>GAMGSKNWFKITIPYGRKYDKAWLLSMIQSKCSVPFTPIEFHYENTRAQFFVEDASTASALKAVNYKILDRENRRISIIINSSAPPHTILNELKPEQVEQLKLIMSKRYDGSQQALDLKGLRSDPDLVAQNIDVVLNRRSCMAATLRIIEENIPELLSLNLSNNRLYRLDDMSSIVQKAPNLKILNLSGNELKSERELDKIKGLKLEELWLDGNSLCDTFRDQSTYISAIRERFPKLLRLDGHELPPPIAFDVEAPTTLPPCKGSYFGTENLKSLVLHFLQQYYAIYDSGDRQGLLDAYHDGACCSLSIPFIPQNPARSSLAEYFKDSRNVKKLKDPTLRFRLLKHTRLNVVAFLNELPKTQHDVNSFVVDISAQTSTLLCFSVNGVFKEVDGKSRDSLRAFTRTFIAVPASNSGLCIVNDELFVRNASSEEIQRAFAMPAPTPSSSPVPTLSPEQQEMLQAFSTQSGMNLEWSQKCLQDNNWDYTRSAQAFTHLKAKGEIPEVAFMK[4x];>[4x]MASVDFKTYVDQACRAAEEF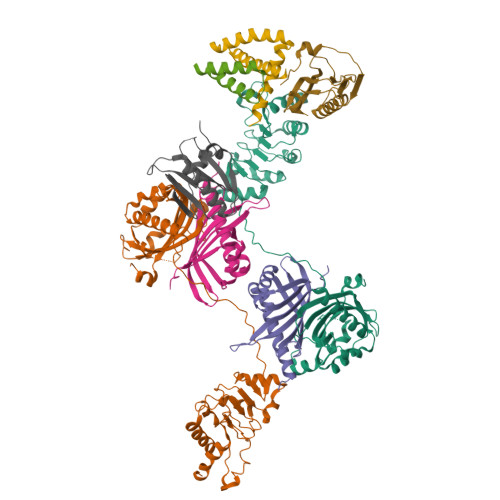VNVYYTTMDKRRRLLSRLYMGTATLVWNGNAVSGQESLSEFFEMLPSSEFQISVVDCQPVHDEATPSQTTVLVVICGSVKFEGNKQRDFNQNFILTAQASPSNTVWKIASDCFRFQDWAS;>GAMGSMDSNTVSSFQVDCFLWHVRKQVADQELGDAPFLDRLRADQASLKGRGSTLGLNIETATCVGKQIVERILKEE[4x];>[4x]SDEAFKMPASRYLTDMTIEEMSRDWFMLMPKQKVAGPLCVRMDQAIMDKNIILKANFSVIFDRLETLTLLRAFTEEGAIVGEISPLPSLPGHTNEDVKNAIGVLIGGLEWNDNTVRVSETLQRFAWRSSNENGGPPLTPTQKRKMAGTIRSEV(2E)-3-[(4-hydroxy-2-oxobutyl)amino]prop-2-enal 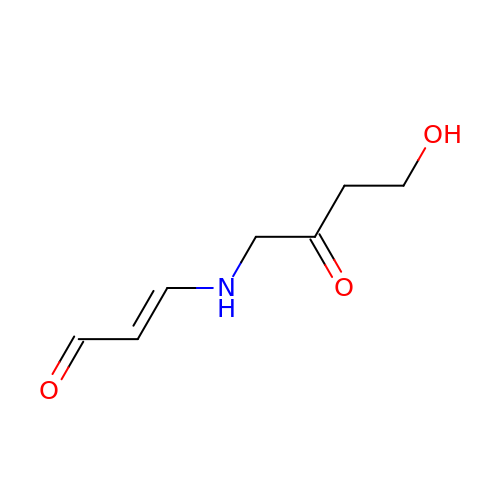| C7 H11 N O3 | WWFGWBHKRFILGQ-HNQUOIGGSA-N>WDGKEDGTGTHSVIVTQAIEMLKHDLSKDEPEAIRNDLSILEKNLHKFQLGSTFPDYDPNAYSLYQDHFWDPDTDHNFTQDNKWYLSYAVPDNAESQTRKFATLAKNEWDKGNYEKAAWYLGQGMHYFGDLNTPYHAANVTAVDSPGHVKFETYAEERKDTYRLDTTGYNTDDAFYKDTLKNDNFNEWSKGYCKYWAKKAKNLYYSHATMSNSWDDWEYAASHGVGNAQKGVAGYLYRFLNDVSNKDAVDKDYDLNEIVVMIKTADVQDAGTDNYIYFGIETKDGVKEEWALDNPGNDFTRNQEGTYTLKLKNKNTKYSDIKNMWIRDEKLTVATD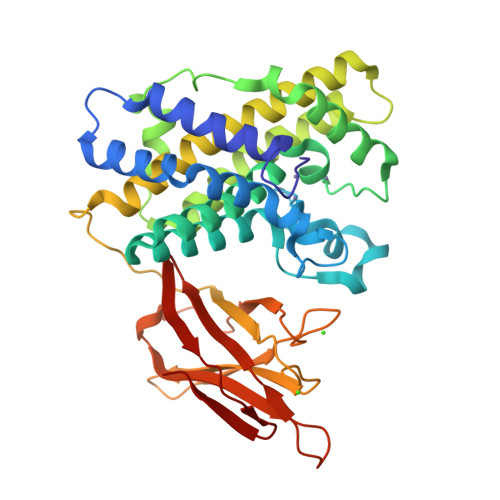GWKPSYVKVIAGDKVRLEKNINEWISGGTTYTLK[4x]>[3x]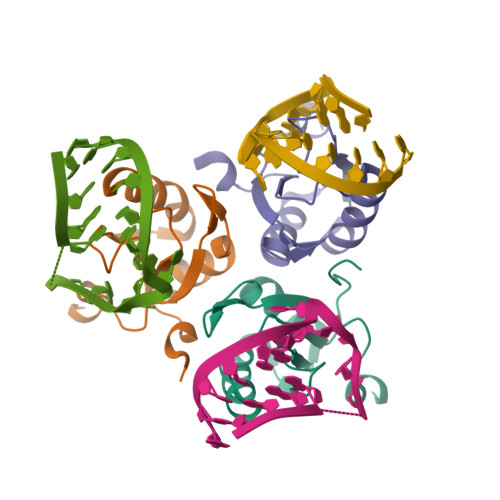AVPETRPNHTIYINNLNEKIKKDELKKSLHAIFSRFGQILDILVSRSLKMRGQAWVIFKEVSSATNALRSMQGFPFYDKPMRIQYAKTDSDIIAKMK> MAHHHHHHMSANNVLVVGGAGFIGSHTAKLLAGQGYAPVVYDNLSTGHQSAVRWGDFVEGDILDQARLVETMEKYAPVAVIHFAASAYVGESVEDPAKYYRNNVGGTQSLLDACRLTRTQNVIFSSSCATYGVPSRLPIGEGEAQNPINPYGRTKLIAEHMLADYAVAYGLRYVALRYFNASGADIDGELGEKHDPETHLIPRAMMAAAGRLDVLEVYG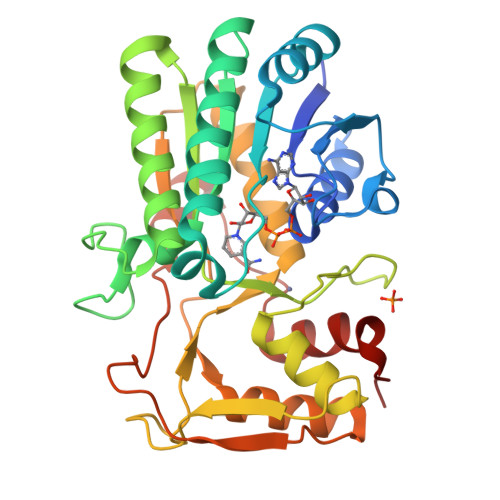DDYETPDGTCIRDYIHVTDLARAHVLAVEHLKEAGGNLAVNLGTGRGTSIREIVQSIGRLTGRSVPVAMRARRAGDPPALYADPALAAEKLGFHTVYSDLDTIIRTAAPHFGLEVRG>MLGAIAYTGNKQSLLPELKSHFPKYNRFVDLFCGGLSVSLNVNGPVLANDIQEPIIEMYKRLINVSWDDVLKVIKQYKLSKTSKEEFLKLREDYNKTRDPLLLYVLHFHGFSNMIRINDKGNFTTPFGKRTINKNSEKQYNHFKQN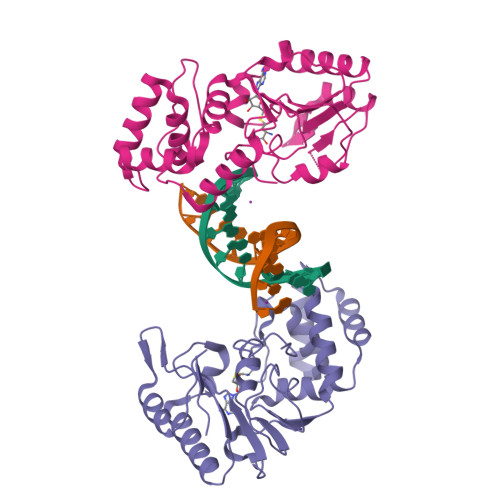CDKIIFSSLHFKDVKILDGDFVYVDPPYLITVADYNKFWSEDEEKDLLNLLDSLNDRGIKFGQSNVLEHHGKENTLLKEWSKKYNVKHLNKKYVFNIYHSKEKNGTDEVYIFN[2x]> GAMAVPDDDDDDDNSNDESEYE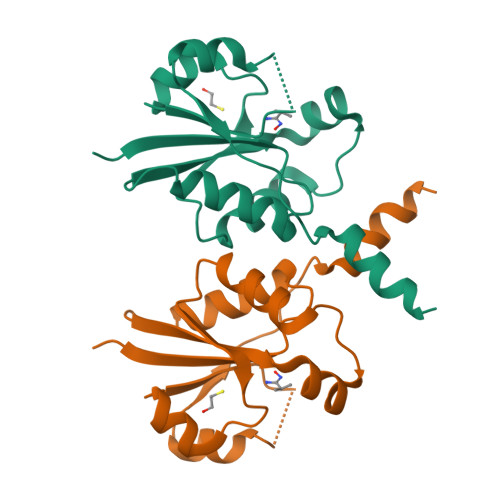SSQMDSEKNKGSIKNSKNVVIYADGVYDMLHLGHMKQLEQAKKLFENTTLIVGVTSDNETKLFKGQVVQTLEERTETLKHIRWVDEIISPCPWVVTPEFLEKYKIDYVAHDDIPYANNQKEDIYAWLKRAGKFKATQRTEGVSTTDLIVRILKNYED verinurad | C20 H16 N2 O2 S | 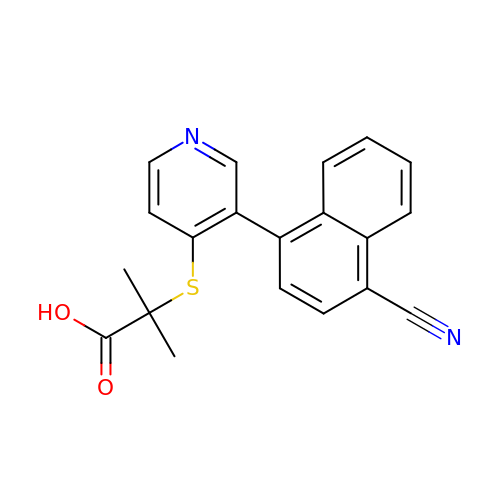YYBOLPLTQDKXPM-UHFFFAOYSA-N~{N}1,~{N}3-bis[4-[[(4~{R})-4-[[4-[[3,5-bis(bromanyl)phenyl]methoxy]phenyl]sulfonylamino]-5-(oxidanylamino)-5-oxidanylidene-pentyl]amino]-4-oxidanylidene-butyl]benzene-1,3-dicarboxamide 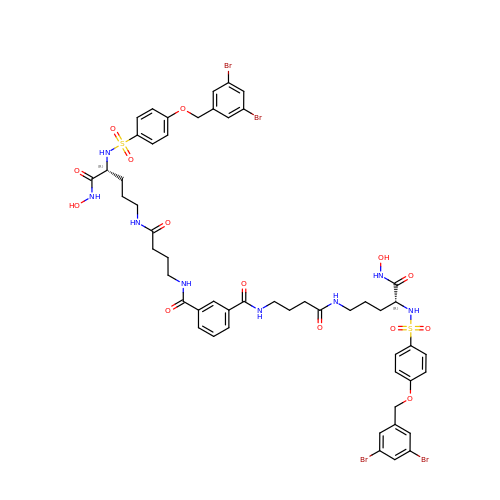| C52 H58 Br4 N8 O14 S2 | JQLHAXGMYALIFJ-AWSIMMLFSA-N>[2x]MQRLEVREPVPYPILVGEGVLKEVPPLAGPAALLFDRRVEGFAQEVAKALGVRHLLGLPGGEAAKSLEVYGKVLSWLAEKGLPRNATLLVVGGGTLTDLGGFVAATYLRGVAYLAFPTTTLAIVDASVGGKTGINLPEGKNLVGAFHFPQGVYAELRALKTLPLPTFKEGL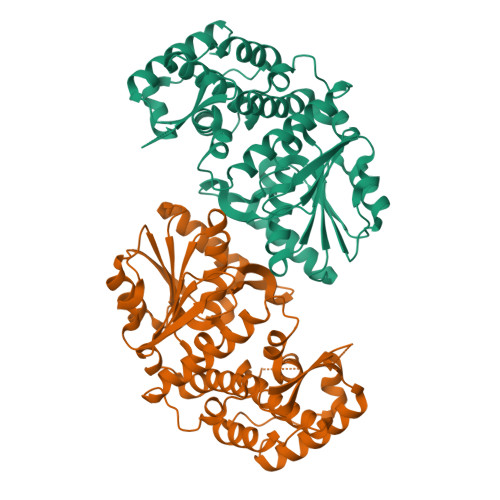VEAFKHGLIAGDEALLKVEDLTPQSPRLEAFLARAVAVKVRVTEEDPLEKGKRRLLNLGHTLGHALEAQTRHALPHGMAVAYGLLYAALLGRALGGEDLLPPVRRLLLWLSPPPLPPLAFEDLLPYLLRDKKKVSESLHWVVPLAPGRLVVRPLPEGLLREAFAAWREELKGLGLLR(1R,4aS,5S,6S,8aR)-5-{[(5S)-1-(3-O-acetyl-4-O-carbamoyl-6-deoxy-2-O-methyl-alpha-L-talopyranosyl)-4-hydroxy-2-oxo-5-(propan-2-yl)-2,5-dihydro-1H-pyrrol-3-yl]carbonyl}-6-methyl-4-methylidene-1,2,3,4,4a,5,6,8a-octahydronaphthalen-1-yl 2,6-dideoxy-3-C-[(1S)-1-{[(3,4-dichloro-5-methyl-1H-pyrrol-2-yl)carbonyl]amino}ethyl]-beta-D-ribo-hexopyranoside | C44 H60 Cl2 N4 O14 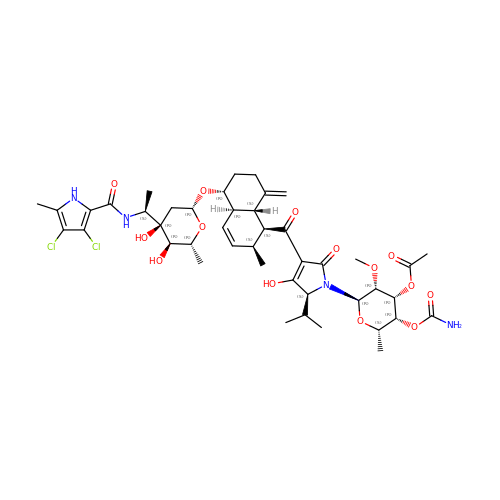| QOFXLOGWNULKEG-FHIRBROQSA-N>[2x]NTKYNKEFLLYLAGFVDGDGSIIAQIKPNQSYKFKHQLSLTFQVTQKTQRRWFLDKLVDEIGVGYV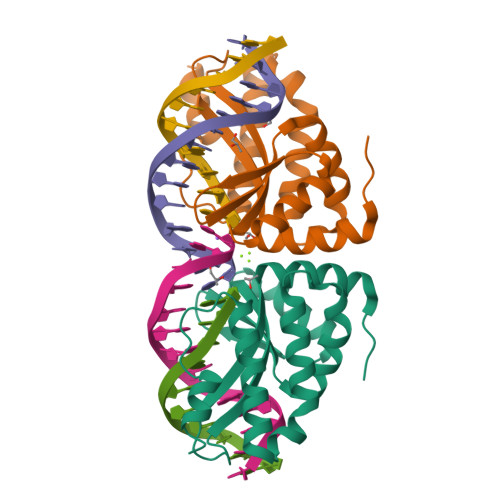RDRGSVSNYILSEIKPLHNFLTQLQPFLKLKQKQANLVLKIIEQLPSAKESPDKFLEVCTWVDQIAALNDSKTRKTTSETVRAVLD> MMQQSRPASDPQVVEAARKEGRLIIYSSTDQSSAQALLDDFRKLYPFIQIEYNDLGTQAIYDRFVSETAAGASSADLLWSSAMELQVKLASEGYALPYDSPEA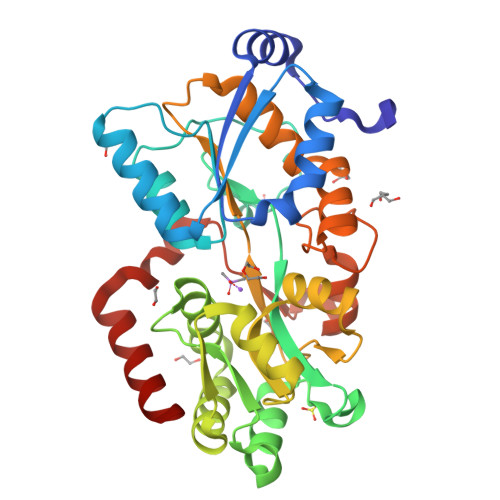KNWPANARLGNLAYSTTLEPAVVVYNKRFLKPEEVPTTREGLARLLQEPRMRGRVATWDPERSAVGFTILKADYDRFPAFQELARAFGKAQAALYSSTGAAFEKVISGEHYLAYGFFGSAALLRQRTVKDLGIAYLTDGTVAIQRVAFINKRAAHPNAAKLFLDYLLSLRGQNLMAYTALIFARRETVVGEATPQALYKAVGGKDKVYAIPVSTEILKNLDPAERMRFLTFWRQAVRGQ> MEKKEFHIVAETGIHARPATLLVQTAS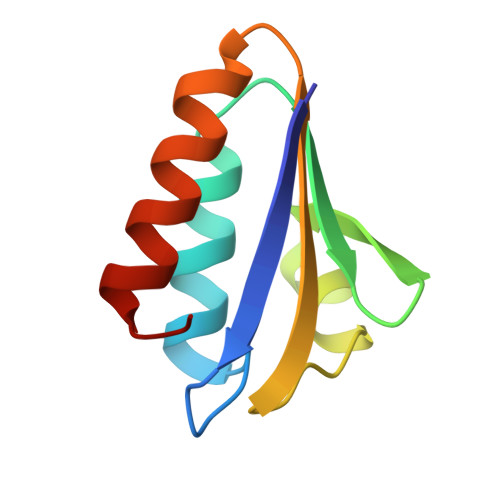KFNSDINLEYKGKSVNLKSIMGVMSLGVGQGSDVTITVDGADEAEGMAAIVETLQKEGLAE3-[5-(1H-IMIDAZOL-1-YL)-7-METHYL-1H-BENZIMIDAZOL-2-YL]-4-[(PYRIDIN-2-YLMETHYL)AMINO]PYRIDIN-2(1H)-ONE 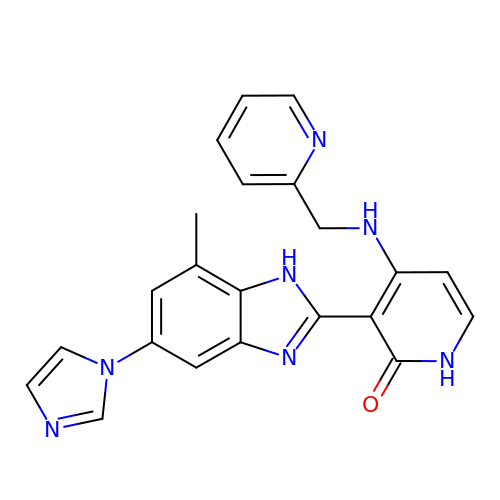| C22 H19 N7 O | GLTRPHMPCVLOJS-UHFFFAOYSA-N>MRAVHLLALGAGLAAASPALANESVLKGVANPAEQVLQTVDYANTRYSKLDQINASNVKNLQVAWTFSTGVLRGHEGSPLVVGNIMYVHTPFPNIVYALDLDQGAKIVWKYEPKQDPSVIPVMCCDTVNRGLAYADGAILLHQADTTLVSLDAKSGKVNWSV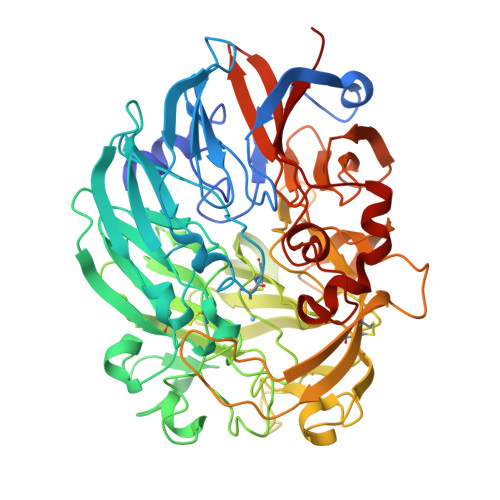KNGDPSKGETNTATVLPVKDKVIVGISGGEFGVQCHVTAYDLKSGKKVWRGYSIGPDDQLIVDPEKTTSLGKPIGKDSSLKTWEGDQWKTGGGCTWGWFSYDPKLDLMYYGSGNPSTWNPKQRPGDNKWSMTIWARNPDTGMAKWVYQMTPHDEWDFDGINEMILTDQKFDGKDRPLLTHFDRNGFGYTLDRATGEVLVAEKFDPVVNWATKVDLDKGSKTYGRPLVVSKYSTEQNGEDVNSKGICPAALGTKDQQPAAFSPKTGLFYVPTNHVCMDYEPFRVTYTPGQPYVGATLSMYPAPGSHGGMGNFIAWDNLQGKIKWSNPEQFSAWGGALATAGDVVFYGTLEGFLKAVDSKTGKELYKFKTPSGIIGNVMTYEHKGKQHVAVLSGVGGWAGIGLAAGLTDPNAGLGAVGGYAALSSYTNLGGQLTVFSLPNN[2x]>MEMENKRSTQKVSRSIPERVKSALWSITAGRCEICCKKLYISDVTGSLVNISQMAHIKAFSPKGPRYSDEENNPHQLDNLLLLCAEHHKMIDTDPDDFPVDWLIKQKKEFEEKVDAVIDTQRIKSSILSFNSIITKNDEIKNEEAEFPKVLLFNDNYFDGNIYRINNALSGIEHDPMYYDLMCQSMKQQIEKIKIPLNSSETISVFAIAPQPLLLYLGYLLNDETNIKIYQRFRTGNLKWNWESSEITNNFYVEQLYTDGNEIDTEVNLILSLSAEISLDRIPTFSNQEYKVPTLILRSDRQGFDAIKSNEDVNEYISVFRNLVVEKIRNDFPNLKCINIFPATPVSVPVRMGMNYQKNIDVEWKIFNQQTNVGFIYSLSLKGEV[4x]

Here, we present the biochemical and structural characterization of two CBASS systems, composed of CdnG and Cap5, from Asticcacaulis sp. and Lactococcus lactis. We show that CdnG from Asticcacaulis sp. synthesizes 3′,2′-cGAMP in vitro, and 3′,2′-cGAMP is the biological signaling molecule that activates Cap5 for DNA degradation. Each monomer of Cap5 is composed of the N-terminal HNH domain, the C-terminal SAVED domain, and a short flexible linker connecting these two domains. The structures revealed that both Cap5 form homodimers, resulting from the side-by-side packing of two HNH domains.

The overall structures of LlCap5 and AsCap5 are very different. The different locations of two SAVED domains are responsible for the difference, as the overall structures of the HNH homodimers are similar. In the structure of LlCap5 homodimer, two SAVED domains do not make any contact, and they are far away from each other. Therefore, the structure of LlCap5 can be described as in open configuration. Specifically, a well-coordinated Mg2+ ion is only observed with AsCap5-HNH, and nine residues of LlCap5-HNH near the active site are disordered. Therefore, it is reasonable to conclude that the configuration of LlCap5 shown in Fig. 3a is enzymatically inactive.> GSMR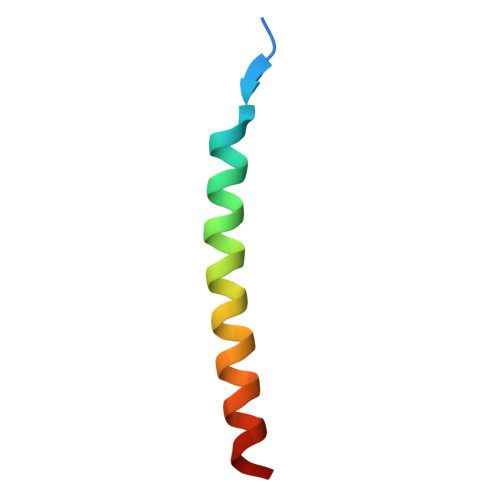MQDATDTVRGLVVELSGLNRLIMSTHRDLEAFKR>[2x]MGSDKIHHHHHHENLYFQGMKRALEFLKECGVFYLATNEGDQPRVRPFGAVFEYEGKLYIVSNNTKKCFKQMIQNPKVEISGMNKKGQWIRLTGEVAND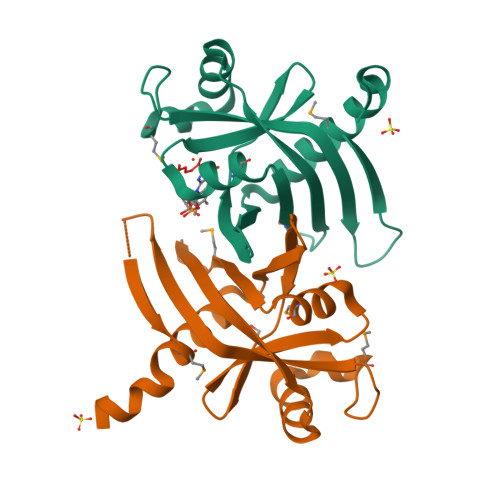DRREVKELALEAVPSLKNMYSVDDGIFAVLYFTKGEGTICSFKGENETFSL>MNIMDFNVKKLAADAGTFLSRAVQFTEEKLGQAEKTELDAHLENLLSKAECTKIWTEKIMKQTEVLLQPNPNARIEEFVYEKLDRKAPSRINNPELLGQYMIDAGTEFGPGTAYGNALIKCGETQKRIGTADRELIQTSALNFLTPLRNFIEGDYKTIAKERKLLQNKRLDLDAAKTRLKKAKAAETRNSSEQELRITQSEFDRQAEITRLLLEGISSTHAHHLRCLNDFVEAQMTYYAQCYQYMLDLQKQLGSFPSNYLSNNNQTSVTPVPSVLPNAIGSSAMASTSGLVITSPSNLSDLKECSGSRKARVLYDYDAANSTELSLLADEVITVFSVVGMDSDWLMGERGNQKGKVPITYLELLN[48x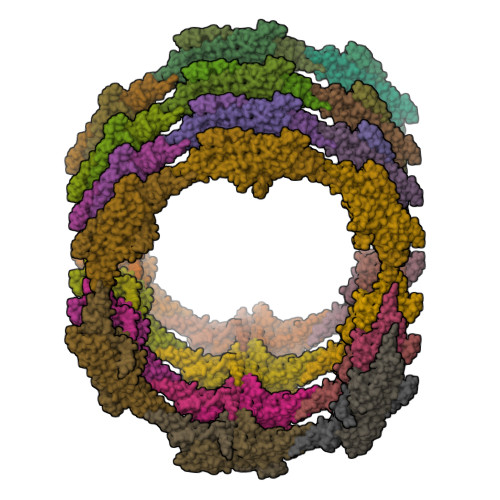]> GPLGSKISKRVNAIEEVNNNVKLLTEMVMSHSQGGAAAGSSEDLMKELYQRCERMRPTLFRLASD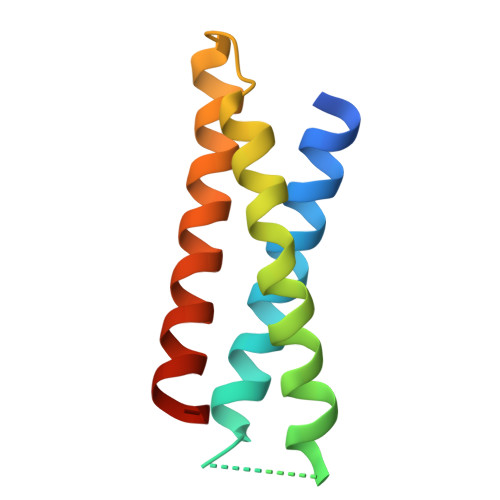TEDNDEALAEILQANDNLTQVINLYKQLVRGEE> SGFTVKPVATVHRRIPDLPDCDIDKWLNNFNVPSPLNWERKIFSNCNFNLSTLLRLVHT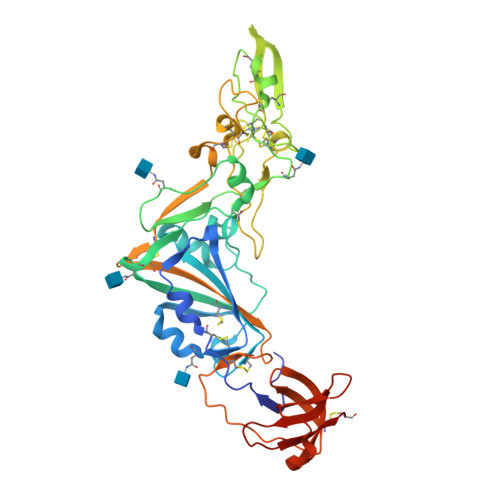DSFSCNNFDESKIYGSCFKSIVLDKFAIPNSRRSDLQLGSSGFLQSSNYKIDTTSSSCQLYYSLPAINVTINNYNPSSWNRRYGFNNFNLSSHSVVYSRYCFSVNNTFCPCAKPSFASSCKSHKPPSASCPIGTNYRSCESTTVLDHTDWCRCSCLPDPITAYDPRSCSQKKSLVGVGEHCAGFGVDEEKCGVLDGSYNVSCLCSTDAFLGWSYDTCVSNNRCNIFSNFILNGINSGTTCSNDLLQPNTEVFTDVCVDYDLYGITGQGIFKEVSAVYYNSWQNLLYDSNGNIIGFKDFVTNKTYNIFPCYAG>[12x]MAKLITLGEILIEFNALSPGPLRHVSYFEKHVAGSEANYCVAFIKQGNECGIIAKVGDDEFGYNAIEWLRGQGVDVSHMKIDPSAPTGIFFIQRHYPVPLKSESIYYRKGSAGSKLSPEDVDEEYVKSADLVHSSGITLAISSTAKEAVYKAFEIASNRSFDTNIRLKLWSAEEAKREILKLLSKFHLKFLITDTDDS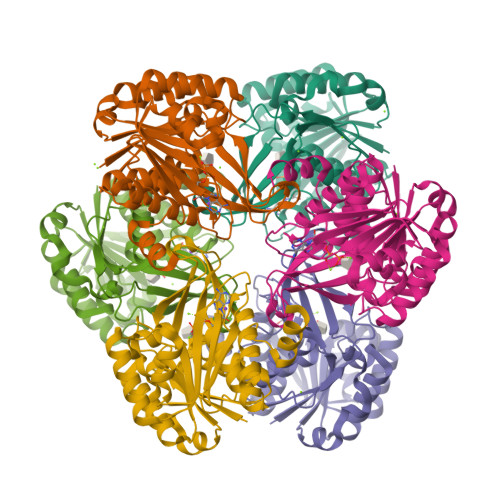KIILGESDPDKAAKAFSDYAEIIVMKLGPKGAIVYYDGKKYYSSGYQVPVEDVTGAGDALGGTFLSLYYKGFEMEKALDYAIVASTLNVMIRGDQENLPTTKDIETFLREMKK> SMSLELQEHCSLKPYNTFGIDVRARLLAHARDEADVREALALARERGLPLLVIGGGSNLLLTRDVEALVLRMASQGRRIVSDAADSVLVEAEAGEAWDPFVQWSLERGLAGLENLSLIPGTVGAAPMQNIGAYGVELKDVFDSLTALDRQDG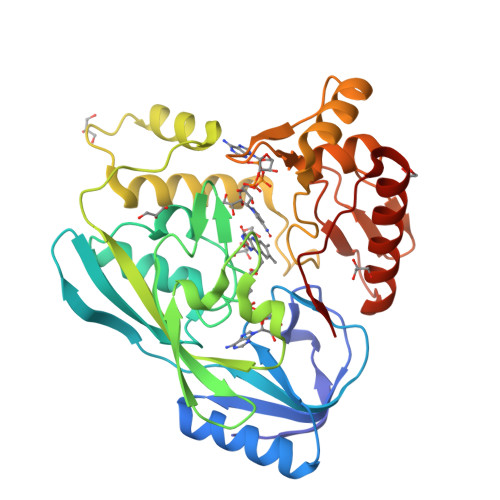TLREFDRQACRFGYRDSLFKQEPDRWLILRVRLRLTRRERLHLDYGPVRQRLEEEGIASPTARDVSRVICAIRREKLPDPAVLGNAGSFFKNPLVDATQAERLRQAFPDLVGYPQADGRLKLAAGWLIDKGGWKGFRDGPVGVHAQQALVLVNHGGATGAQVRALAERIQEDVRRRFGVELEPEPNLY> GGACACGAGUAACUCGUCUAUCUUCUGCAGGCUGCUUACGGUUUCGUCCGUGUUGCAGCCGAUCAUCAGCACAUCUAGGUUUCG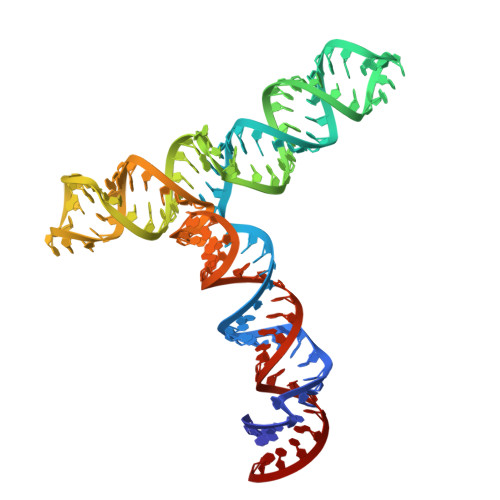UCCGGGUGUGACCGAAAGGUAAGAUGGAGAGCCUUGUCCC ISOPROPYL 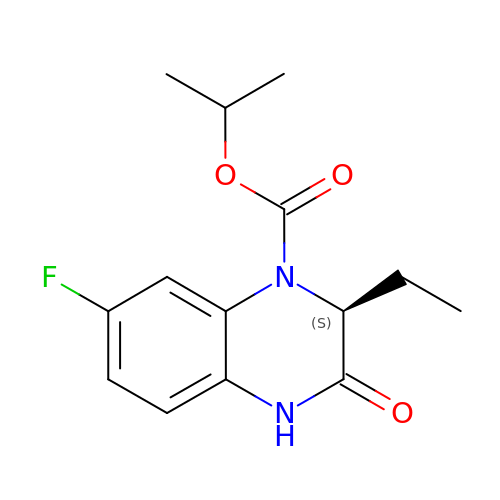(2S)-2-ETHYL-7-FLUORO-3-OXO-3,4-DIHYDROQUINOXALINE-1(2H)-CARBOXYLATE | C14 H17 F N2 O3 | KELNNWMENBUHNS-NSHDSACASA-N> SMHSDLTFCEIILMEMESHDAAWPFLEPVNPRLVSGYRRIIKNPMDFSTMRERLLRGGYTSSEEFAADALLVFDNCQTFNEDDSEVGKAGHIMRRFFESRWEEFYQ

Chromatin remodeling complex NoRC (nucleolar remodeling complex) interacts with the rDNA promoter regions of silent genes repressing rDNA transcription. It consists of TIP5 (TTF-I interacting protein 5), also known as BAZ2A (bromodomain [BRD] adjacent to zinc finger domain protein 2A), which is the largest subunit, and the adenosine triphosphatase (ATPase) SNF2h (sucrose nonfermenting protein 2 homologue). BAZ2B shares 29% sequence identity with TIP5 at the full-length level and harbors similar domain organization. Both proteins contain a MBD (methyl-CpG-binding domain), also known as TAM (TTF-IIP5, ARBP, MeCP1) domain, AT-hook DNA-binding domains, DDT (DNA binding homeobox and different transcription factors), and a PHD (plant homeodomain) zinc finger adjacent to a BRD at their C terminus. Our crystal structures combined with biophysical and mutagenesis data demonstrate that PHD zinc fingers recognize N-terminal unmodified H3K4 tail, whereas the TIP5 and BAZ2B BRDs recognize H4K16ac and H3K14ac, respectively, with specificity pattern KacXXR.

To gain insight into the recognition of acetylation marks by the NoRC complex, we solved crystal structures of the TIP5 BRD in its free form and in complex with a H4K16acK20ac histone peptide and two cocrystal structures of BAZ2B BRD bound to H3K14ac and H4K8acK12ac peptides. The crystal structures of free-state TIP5 BRD as well as in complex with H4K16acK20ac were solved at 1.76 and 1.65 Å resolution, respectively. Interestingly, both TIP5 and BAZ2B BRD contain the aromatic “WPF shelf” at the ZA loop shared with BRD families such as the BET family. However, in the BAZ BRDs, these three aromatic residues adopt a closer conformation compared with the more open form of BET BRDs that creates a wider binding site sufficient to accommodate two acetyl-lysine side chains in BET (Morinière et al., 2009; Filippakopoulos et al., 2012). On the other hand, it has been shown that the tandem PHD finger-BRD modules of human TIP5 represent an independent unit that interacts with H4K16ac and triggers the cascade of events that establish the repressed state of rDNA. Zhou and coworkers reported that inactive TIP5 BRD mutant at the conserved tyrosine does not repress Pol I transcription and suggested that interaction of the BRD with acetylated histone H4 is a key event in NoRC-mediated gene silencing. Isothermal titration calorimetry (ITC) data suggest a preference of the TIP5 BRD for K16ac.> EITCQENLPFTCGNTDALNSSSFSSDFIFGVASSAYQIEGTIGRGLNIWDGFTHRYPNKSGPDHGNGDTTCDSFSYWQKDIDVLDELNATGYRFSIAWSRIIPRGKRSRGVNEKGIDYYHGLISGLIKKGITPFVTLFHWDLPQTLQDEYEGFLDPQIIDDFKDYADLCFEEFGDSVKYWLTINQLYSVPTRGYGSALDAPGRCSPTVDPSCYAGNSSTEPYIVAHHQLLAHAKVVDLYRKNYTHQGGKIGPTMITRWFLPYNDTDRHSIAATERMKEFFLGWFMGPLTNGTYPQIMIDTVGERLPSFSPEESNLVKGSYDFLGLNYYFTQYAQPSPNPVNSTNHTAMMDAGAKLT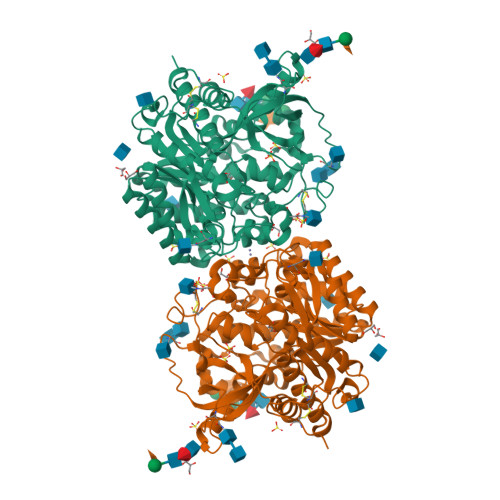YINASGHYIGPLFEKDKADSTDNIYYYPKGIYSVMDYFKNKYYNPLIYVTENGISTPGDENRNQSMLDYTRIDYLCSHLCFLNKVIKEKDVNVKGYLAWALGDNYEFNKGFTVRFGLSYIDWNNVTDRDLKKSGQWYQTFISP> EKQQWFCNSSDAIISYSYCDHLKFP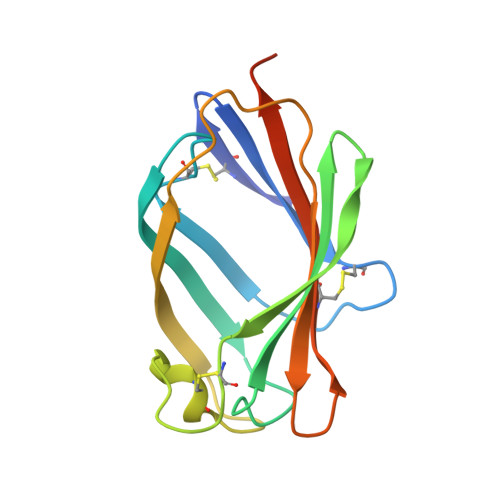ISISSEPCIRLRGTNGFVHVEFIPRGNLKYLYFNLFISVNSIELPKRKEVLCHGHDDDYSFCRALKGETVNTSIPFSFEGILFPKGHYRCVAEAIAGDTEEKLFCLNFTIIHRRDVNKGENLYFQ> TPFPWNKIRLPEYVIPVHYDLLIHANLTTLTFWGTTKVEITASQPTSTIILHSHHLQISRATLRKGAGERLSEEPLQVLEHPRQEQIALLAPEPLLVGLPYTVVIHYAGNLSETFHGFYKSTYRTKEGELRILASTQFEPTAARMAFPCFDEPAFKASFSIKIRREPRHLAISNMPLVKSVTVAEGLIEDHFDVTVKMSTYLVAFIISDFESVSKITKSGVKVSVYAVPDKINQADYALDAAVTLLEFYEDYFSIPYPLPKQDLAAIPDFQSGAMENWGLTTYRE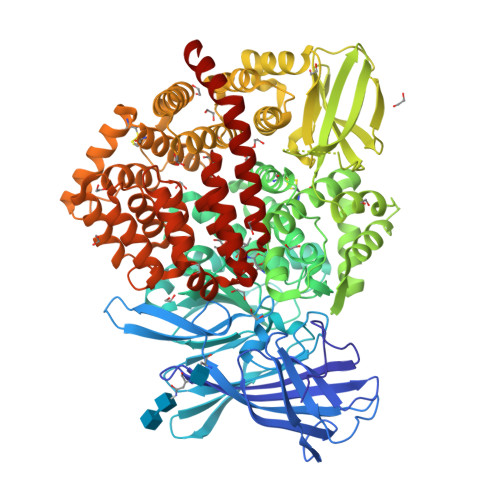SALLFDAEKSSASSKLGITMTVAHELAHQWFGNLVTMEWWNDLWLNEGFAKFMEFVSVSVTHPELKVGDYFFGKCFDAMEVDALNSSHPVSTPVENPAQIREMFDDVSYDKGACILNMLREYLSADAFKSGIVQYLQKHSYKNTKNEDLWDSMASISGDVKTMMNTWTLQKGFPLITITVRGRNVHMKQEHYMKGDTGYLWHVPLTFITSKSDMVHRFLLKTKTDVLILPEEVEWIKFNVGMNGYYIVHYEDDGWDSLTGLLKGTHTAVSSNDRASLINNAFQLVSIGKLSIEKALDLSLYLKHETEIMPVFQGLNELIPMYKLMEKRDMNEVETQFKAFLIRLLRDLIDKQTWTDEGSVSERMLRSQLLLLACVHNYQPCVQRAEGYFRKWKESNGNLSLPVDVTLAVFAVGAQSTEGWDFLYSKYQFSLSSTEKSQIEFALCRTQNKEKLQWLLDESFKGDKIKTQEFPQILTLIGRNPVGYPLAWQFLRKNWNKLVQKFELGSSSIAHMVMGTTNQFSTRTRLEEVKGFFSSLKENGSQLRCVQQTIETIEENIGWMDKNFDKIRVWLQSE>[3x]MQQLNPSEISALIKQRIGDLDTSATAKNEGTIVMVSDGIVRIHGLADAMYGEMIEFDGGLFGMALNLEQDSVGAVVLGNYLSLQEGQKARCTGRVLEVPVGPELLGRVVDALGNPIDGKGPIDAKLTDAVEKVAPGVIWRQSVDQPVQTGYKSVDTMIPVGRGQRELIIGDRQTGKTAMAIDAIIAQKNSGIKCVYVAIGQKQSTIANVVRKLEETGAMAYTTVVAAAAADPAAMQYLAPYSGCTMGEYFRDRGEDALIIYDDLSKQAVAYRQISLLLRRPPGREAYPGDVFYLHSRLLERASRVSAEYVEKFTNGAVTGKTGSLTALPIIETQAGDVSAFVPTNVISITDGQIFLETSLFNAGIRPAVNAGISVSRVGGSAQTKIIKKLSGGIRTALAQYRELAAFAQFASDLDEATRKQLEHGQRVTELMKQKQYAPYSIADQAVSVYASNEGYMADVEVKKIVDFDAALIAYFRSEYAPLMKQIDETGDYNKDIEAAIKAGIESFKATQTY;>[3x]MSSGRIIQIIGAVIDVEFERTSVPKIYDALQVDGTETTLEVQQQLGDGVVRTIAMGSTEGLKRGLTVTSTNAPISVPVGTATLGRIMDVLGRPIDEAGPVATEERLPIHRQAPSYAEQAASTDLLETGIKVIDLLCPFAKGGKVGLFGGAGVGKTVNMMELINNIAKAHSGLSVFAGVGERTREGNDFYHEMKDSNVLDKVAMVYGQMNEPPGNRLRVALTGLTMAEYFRDEKDENGKGRDVLLFVDNIYRYTLAGTEVSALLGRMPSAVGYQPTLAEEMGVLQERITSTKSGSITSIQAVYVPADDLTDPSPATTFAHLDATVVLSRDIASSGIYPAIDPLDSTSRQLDPLVVGQEHYEIARAVQNVLQRYKELKDIIAILGMDELAEEDKLVVYRARKIQRFFSQPFHVAEVFTGAPGKLVPLKETIRGFKGLLAGEYDHIPEQAFYMVGGIDEVIAKAEKL;>MELTLGLVAIASAILIAFGALGTAIGFGLLGGRFLEAVARQPELAPQLQTRMFLIAGLLDAVPMIGVGIGLFFIFANPFVG[10x];> MAAEEHALTSTEYIKHHLTNMTYGKMPDGTWKLAETAEEAHSMGFTAIHLDSMGWSIGLGVIFCLLFWIVARAANAGVPTKFQSAIEMIIEFVDSSVRDTFHGKSRLIAPLALTIFVWIFLMNLMDLIPVDWIPQVAAFVGANVFGMDPHHVYFKIVPSTDPNITLGMSLSVFVLILFYSIREKGVGGFVGELALNPFNPSNPVAKALLIPVNLILELVTFLARPISLALRLFGNMYAGELIFILIALLPFWIQWALSVPWAIFHILVITLQAFIFMMLTIVYLSMASEKH;>[2x]MNINLTLIGQAIAFAFFVAFCMKFVWPPLINAISERQRKIADGLNAAEKAKADLADAQAQVKQELDAAKAQAAQLIEQANRRAAQLIEEARTQAAAEGERIRQQAKEAVDQEINSAREELRQQVAALAVTGAEKILNQQVDAEAHNAMLSQLAAKL;> MAELLTLARPYAKAAFAYASEQGATDNWSNALQVLSAAVQDEAFSAYLNRPELTPAEQVKLFAKVLGEDQSQAVSNFLTLLADNDRLVLLPE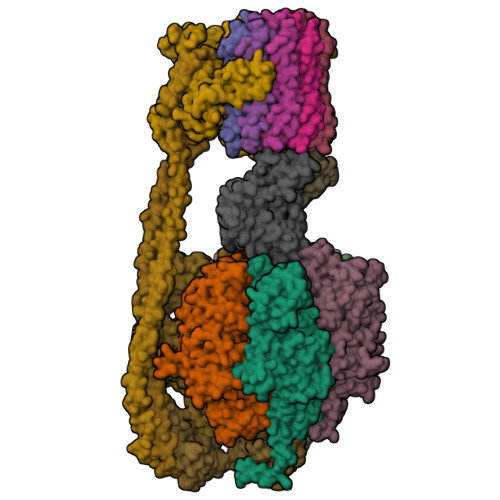IAAEYEQLKSQNNNNVDVVIESAFPLTAEQEQLLKSALEKRFNSTVTVSVEVKPELIAGVVIRAGDQVIDDSALNKLEKMRTRLLA;> MATMQCDVVSVKESIYSGAVTMLIAKGAGGELGILPGHAPLVTLLQPGPIRVLLENGTEEIVYVSGGVLEVQPHVVTVLADTAIRADNLDEAAILEARKNAEQLLANQKSDLDSAAALAALAETAAQLETIRKIKNRAQ;> MANLKEIRAKVASIKSTQKITRAMQMVAASKMRRAQERMAQGRPYADNMRRVIAHLVQANPEYKHRYMVDRPVKRVGYIIVSSDRGLAGGLNINLFKKVVQHVKAQQEQSIEVQFALIGQKAVSFFKNYGGKVLGATTQIGDAPSLEQLTGSVQVMLDAFDKGELDRIYLVSNGFVNAMTQKPKVEQLVPLAPAEEGDDLNRTYGWDYIYEPEAEELLNGLLVRYIESMVYQGVIENVACEQSARMVAMKAATDNAGQLIKDLQLIYNKLRQAAITQEISEIVGGAAAV> EDAFRKLFRFYRQSRPGTADLGAVIDFSEAHLARSPKPGVPQVVRFPLNVSSVTERDAERVGLEPVSKWRAYGLEGYPGFIFIPNPFLPGCQRHWVKQCLKLYSQKPNVSNLDKHMTKEETQGLWEQSKE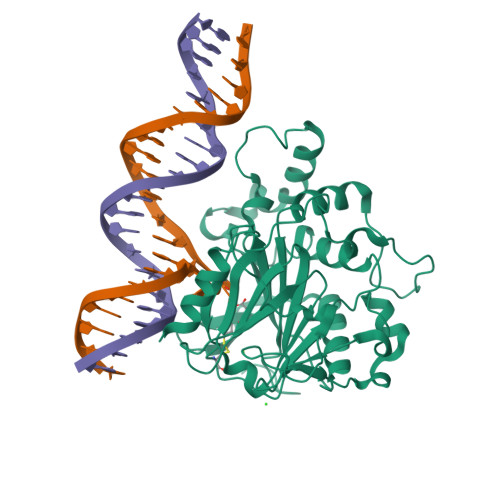VLRSKEVTKRRPRSLLERLRWVTLGYHYNWDSKKYSADHYTPFPSDLAFLSEQVATACGFQGFQAEAGILNYYRLDSTLGIHVDRCELDHSKPLLSFSFGQSAIFLLGGLKRDEAPTAMFMHSGDIMVMSGFSRLLNHAVPRVLPHPDGESLPHSLETPLPAVLPSNSLVEPSSVEDWQVCATYLRTARVNMTVRQVLATGQDFPL> GKPLHEQLWYHGAIPRAEVAELLVHSGDFLVREGQSQPDYVLSVLWDGLPRHFIIQSLDNLYRLEGEGFPSIPLLIDHLLSTQQPLTK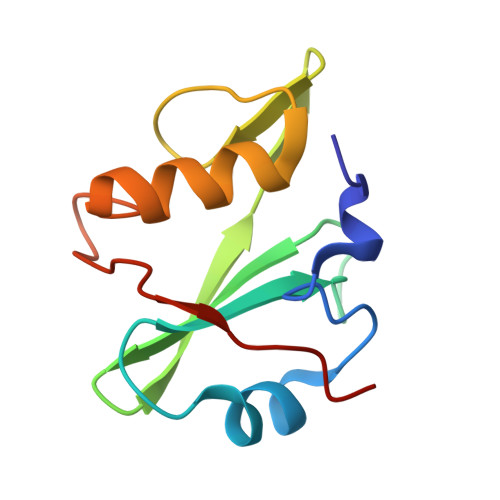KSGVVLHRAVPKSRA Polymerases generate nascent strands of genetic material by stepwise phosphoryl transfer of nucleotides to primer termini, yielding O3′→P5′ phosphodiester linkages. We reported that 3′-NH2 primer extension can be catalyzed by a modified DNA polymerase, yielding N3′→P5′ phosphoramidate DNA (NP-DNA). The large fragment of DNA polymerase I (BF), cloned from the thermophilic soil bacterium Geobacillus stearothermophilus (Bst), acquires nontrivial levels of N3′→P5′ polymerase activity via two surprisingly minor substitutions: (A) a single active site mutation (F710Y) and (B) substitution of its divalent Mg2+ cofactors with Ca2+ (1). To add evidence that a single divalent metal ion cofactor catalyzes unnatural NP synthesis in BF, a polymerase A family member, we carried out a single nucleotide primer extension reaction in intact crystals.

Reactions were then initiated in the intact crystals by pH-shift from an acidic mother liquor (pH < 6) to a basic soaking liquor at pH 8.8, and reacting crystals were quenched at various times by flash freezing. Early time points show negligible differences in ordered density between the ground state complex crystallized under acidic conditions versus the complex after 1 h of soaking under reaction conditions, suggesting that the reactant state and ground state cannot be clearly distinguished in this resolution range. Conformational changes in both the upstream and downstream nucleotides flanking the nascent bond are linearly correlated with covalent bonding. The downstream conformational change in the dGTP substrate sugar from C2′- to C3′-endo upon product formation, however, was not observed in an equivalent time-resolved experiment with the wild-type enzyme, in which the conformation is stably C3′-endo. The lack of electron density for an A-site metal ion in the ground state and at later time points is also consistent with the expectation of a neutral nucleophile in the NP reaction and the generally weak affinity of aliphatic amines for Ca2+. Unlike for native phosphodiester catalysis, only a single metal ion cofactor is detectable by crystallography during NP catalysis.

>[2x]KMAFTLADRVTEEMLADKAALVVEVVEENYHDAPIVGIAVVNEHGRFFLRPETALADPQFVAWLGDETKKKSMFDSKRAAVALKWKGIELCGVSFDLLLAAYLLDPAQGVDDVAAAAKMKQYEAVRPDEAVYGKGAKRAVPDEPVLAEHLVRKAAAIWELERPFLDELRRNEQDRLLVELEQPLSSILAEMEFAGVKVDTKRLEQMGKELAEQLGTVEQRIYELAGQEFNINSPKQLGVILFEKLQLPVLKKTKTGYSTSADVLEKLAPYHEIVENILHYRQLGKLQSTYIEGLLKVVRPATKKVHTIFNQALTQTGRLSSTEPNLQNIPIRLEEGRKIRQAFVPSESDWLIFAADYSQIELRVLAHIAEDDNLMEAFRRDLDIHTKTAMDIFQVSEDEVTPNMRRQAKAVNFGIVYGISDYGLAQNLNISRKEAAEFIERYFESFPGVKRYMENIVQEAKQKGYVTTLLHRRRYLPDITSRNFNVRSFAERMAMNTPIQGSAADIIKKAMIDLNARLKEERLQAHLLLQVHDELILEAPKEEMERLCRLVPEVMEQAVTLRVPLKVDYHYGSTWYDAK(2R)-3-{[(S)-(2-aminoethoxy)(hydroxy)phosphoryl]oxy}-2-(tetradec-5-enoyloxy)propyl 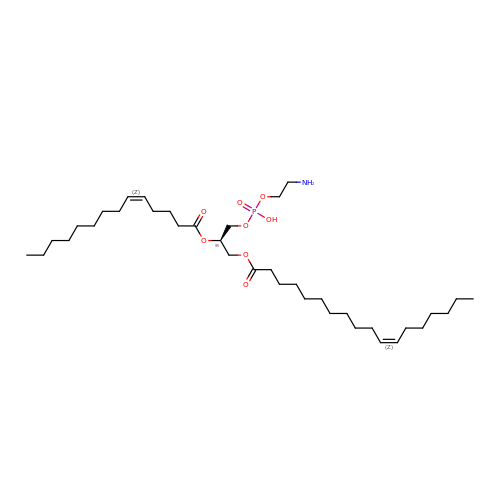(11Z)-octadec-11-enoate | C37 H70 N O8 P | SWNDXEVFPWKPGK-SPZKJSGBSA-N>MKMFFRLTRELRDELKRPLGELVRGPIPEPYLKVRGELEKHPVVTVGDVVTENVLKIGVKPIIALYDLKTKRKEYSPEIEDTAVFLTVTNPPGTITKALLDTVRKAFGLAERGRNVHILVSGEEDLAAIPAVLYAPLGTLVLYGQPDEGVVLIKVTPEC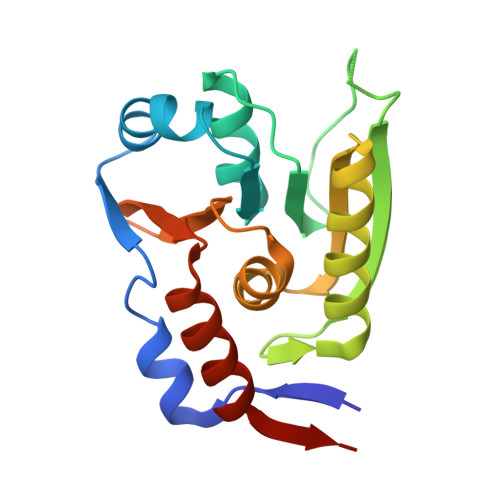KRRCAKILASMEVVRDGD[2x]> STSKDHVKSQIPRLSAINDLHKIWPTVEEHGAAIIESFLSLDIVRRLNEEVDPFVKIEPIPAAKTKDHPNHKLSTTTRLVNVLAPISKAYREDVLNSKVLHRICSDAFHVYGDYWVLMGAVMELAPSNPAQPLHRDMRFSHPIVEYLKPDAPATSINFLVALSPFTAENGATHVILGSHKWQNLSNVSMDATVRALMNPGDALLITDSTIHCGGAETTGTETRRLLTITMGISQLTPLESNLAVPRPVIESLTPLAQRLLGWASQRSAAPRDIGLLTIRGNSIEKTMNLKAEQPLHDDE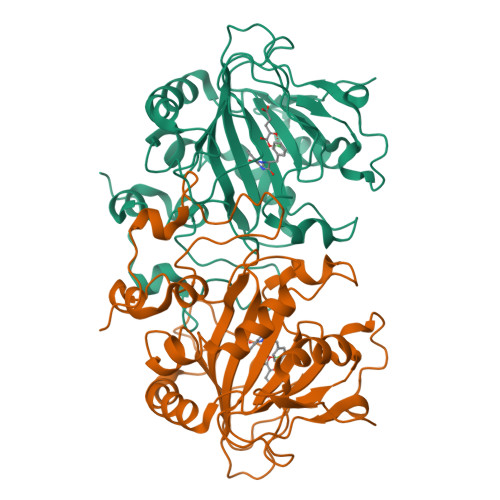AEPLCRETI[5-(6-aminopurin-9-yl)-2-(hydroxymethyl)furan-3-yl] [5-(6-aminopurin-9-yl)-3-oxidanyl-furan-2-yl]methyl hydrogen phosphate | C20 H17 N10 O8 P | 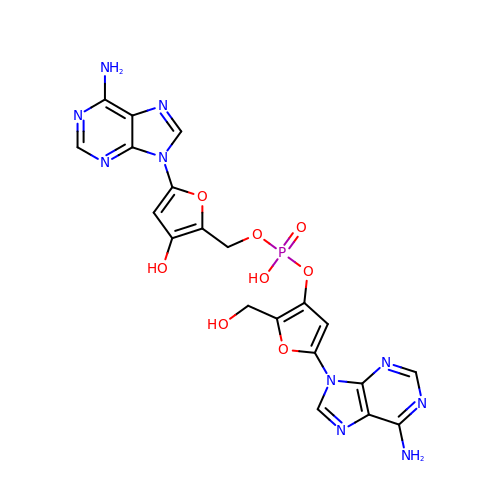XKEWDTWLEZMIAN-UHFFFAOYSA-N The E. coli Paraquat Inducible (Pqi) Pathway is a putative Gram-negative phospholipid transport system. The pathway comprises three components: an integral inner membrane protein (PqiA), a periplasmic spanning MCE family protein (PqiB) and an outer membrane lipoprotein (PqiC). PqiC is predicted to anchor within the periplasmic face of the OM and comprises an ABC auxiliary lipoprotein domain (formerly DUF330). Interactions between all complex components, including stoichiometry, remain uncharacterised; nevertheless, once assembled into their quaternary complex, the trio of Pqi proteins are anticipated to provide a continuous channel between the inner and outer membranes of diderms.

Consequently, we designed a second N-terminally truncated construct, in which residues 1–16 were replaced with a hexa-histidine tag and TEV protease recognition site, referred to as PqiC17-187, which was expressed cytoplasmically. After TEV cleavage of the N-terminal hexa-histidine tag, the sequence of PqiC17-187 differed from the native processed PqiC lipoprotein only by the removal of the N-terminally acylated Cysteine (C16). We therefore propose PqiC17-187 to purify as a monomeric species in contrast to the octameric oligomer of PqiC, implying multimerisation is dependent upon the N-terminal lipidated moiety. The PqiC17-187 structure, solved to 2.1 Å, displayed an arrangement unique to that observed in the PqiC structure with three copies present within the asymmetric unit. Two of these chains, chains A and B, sit in orientations similar to those of the two corresponding chains in the native PqiC asymmetric unit, however, the third chain, Chain C, sits perpendicular and slightly below the plane of the other two, interfacing with the bottom corner of chain A. Despite this global geometry change, the monomers from each structure align strongly yielding an RMSD of 0.568 Å across 151 pruned atom pairs and 0.591 Å across all 152 pairs. Whilst the density corresponding to the first residues of the β1-β2 loop region (residues 27–31) is more clearly resolved than in the full length PqiC structure, the electron density for the extremity of the loop (residues 32–44) was mostly absent from the 2mFo – DFc map contoured at 1 sigma preventing modelling of this region. Despite this, the electron density corresponding with the core of the protein was a considerable improvement over that of the full length PqiC structure with side chain information clearly defined in both β-sheet and α-helical regions. Overall, our PqiC17-187 structure provided us with high-resolution side chain information throughout PqiC, with the exception of the β1-β2 loop region, confirming the conformation of key residues of interest lining the octameric pore. Consequently, PqiC17-187 monomers are able to adopt a conformation more favourable for crystal packing thus, the molecules within the unit cell no longer assemble an octameric structure.

>[3x]QMSSGEINKNYYQLPVVQSGTQSTASQGNRLLWVEQVTVPDYLAGNGVVYQTSDVKYVIANNNLWASPLDQQLRNTLVANLSTQLPGWVVASQPLGSAQDTLNVTVTEFNGRYDGKVIVSGEWLLNHQGQLIKRPFRLEGVQTQDGYDEMVKVLAGVWSQEAASIAQEIKRLP>[2x]MDREPQHEELPGLDSQ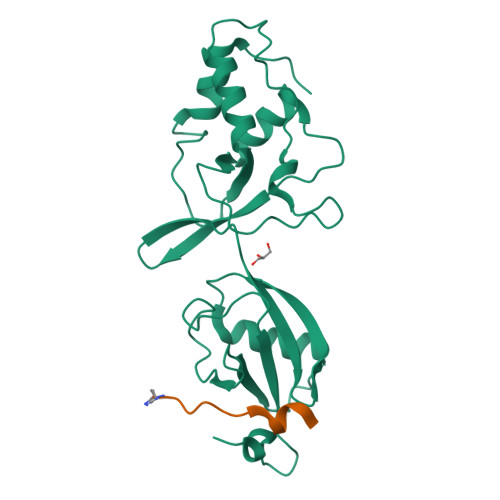WRQIENGESGRERPLRAGESWFLVEKHWYKQWEAYVQGGDQDSSTFPGCINNATLFQDEINWRLKEGLVEGEDYVLLPAAAWHYLVSWYGLEHGQPPIERKVIELPNIQKVEVYPVELLLVRHNDLGKSHTVQFSHTDSIGLVLRTARERFLVEPQEDTRLWAKNSEGSLDRLYDTHITVLDAALETGQLIIMETRKKDGTWPSAQLEHHHHHH;>[2x]AEGEFYKLKIRTPR> GSMAEQVTKSVLFVCLGNICRSPIAEAVFRKLVTDQNISENWRVDSAATSGYEIGNPPDYRGQSCMKRHGIPMSHVARQITKEDFATFDYILCMDESNLRDLNRKSNQVKTCKAKIELLGSYDPQKQLIIE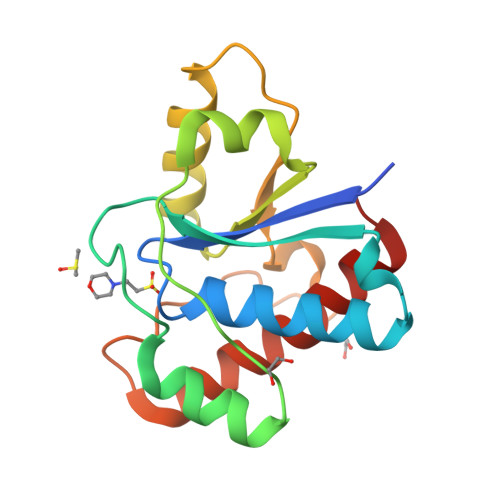DPYYGNDSDFETVYQQCVRCCRAFLEKAH>[5x]MVQTSFEHHHHHHSAGENLYFQGAQISMNIKLEIQKMAKEIGISKIGFTTADDFDYLEKSLRLGVEEGRTTGFEHKNIEERIYPKLSLESAKTIISIAVAYPHKLPQQPQKTEFKRGKITPNSWGLDYHYVLQDKLKRLAKGIEKLTENFEYKGMVDTGALVDTAVAKRAGIGFIGKNGLVISKEYGSYMYLGELITNLEIEPDQEVDYGCGDCRRCLDACPTSCLIGDGTMNARRCLSFQTQDKGMMDMEFRKKIKTVIYGCDICQISCPYNRGIDNPLASDIDPDLAMPELLPFLELTNKSFKETFGMIAGSWRGKNILQRNAIIALANLHDRNAIVKLMEIIDKNNNPIHTATAIWALGEIVKKPDEGMLDYMRGLSPKDEHSQAEWELVCAKWQI

Queuosine (Q) is a hypermodified RNA base that replaces guanine in the wobble positions of 5′-GUN-3′ tRNA molecules. The final step in Q biosynthesis is the reduction of the epoxide precursor, epoxyqueuosine, to yield the Q cyclopentene ring. The epoxyqueuosine reductase responsible, QueG, shares distant homology with the cobalamin-dependent reductive dehalogenase (RdhA), however the role played by cobalamin in QueG catalysis has remained elusive. We report the solution and structural characterization of Streptococcus thermophilus QueG, revealing the enzyme harbors a redox chain consisting of two [4Fe-4S] clusters and a cob(II)alamin in the base-off form, similar to RdhAs.

We subsequently repeated protein preparation, crystallization, and crystal harvesting under anaerobic conditions, leading to significantly improved x-ray diffraction. The anaerobic QueG crystal structure contains 5 monomers in the asymmetric unit (AU). No obvious differences can be observed between the individual molecules, with an r.m.s.d. between monomers ranging from 0.1–0.2 Å. Electron density for the three redox cofactors is well defined, with the corrin plane located at the bottom of a deep surface pocket, providing direct access to the cobalt ion from the solvent. The cobalamin is bound in a pentacoordinate, base-off form by a nitroreductase-type module, similar to what is observed for the reductive dehalogenases and the distantly related vitamin B12 processing enzyme CblC. The closest Fe-Fe distance between both [4Fe-4S] sulfur clusters is 9.5 Å in QueG, compared with 9.3 Å for the S. multivorans RdhA. In QueG, high levels of disorder can be observed for a loop region connecting two of the cysteine ligands (Cys-184 and Cys-187) to the first [4Fe-4S] cluster, suggesting the possibility of ligand heterogeneity for this particular cofactor. One side of the active site cavity is markedly more hydrophilic compared with the opposite face, and consists of the strictly conserved D100-Y101-H102 QueG motif in addition to the conserved D130. A putative salt bridge network is observed between D100-H102 and Asp-130, the latter residue pointing directly toward the cobalt fifth ligand region. Tyrosine 101 is located adjacent to D130 and similarly points directly to the cobalt water ligand, although neither is close enough to establish direct hydrogen bonds (both at ∼4.0 Å distance from the cobalt water ligand).4-methyl-6-(2-{3-[3-(methylamino)propyl]phenyl}ethyl)pyridin-2-amine 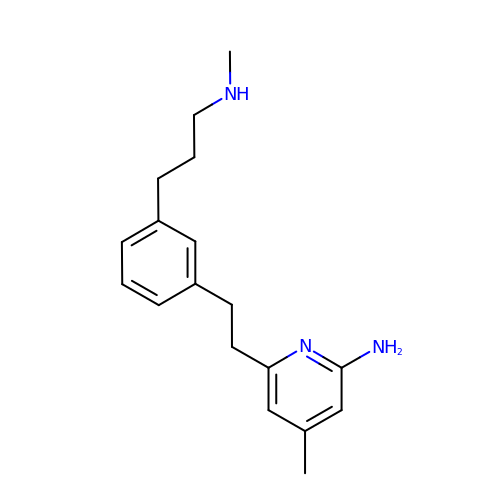| C18 H25 N3 | CUTMJYPBBFYFJH-UHFFFAOYSA-N(4'-{[ALLYL(METHYL)AMINO]METHYL}-1,1'-BIPHENYL-4-YL)(4-BROMOPHENYL)METHANONE 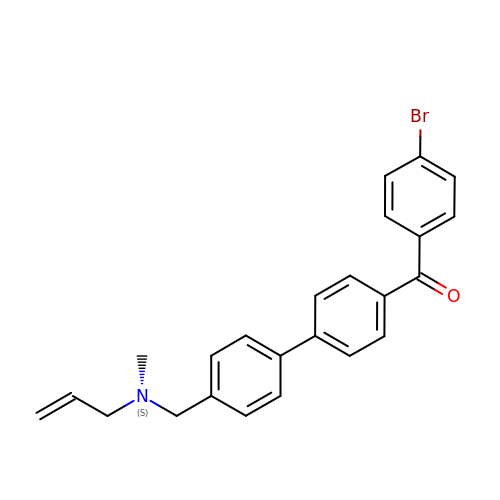| C24 H22 Br N O | YATCZCSDJCQNAL-UHFFFAOYSA-N{4-[2-(5-fluoro-2-{3-[(methylamino)methyl][1,2,4]triazolo[4,3-a]pyridin-6-yl}phenoxy)ethyl]-1,5-dimethyl-1H-pyrazol-3-yl}(morpholin-4-yl)methanone 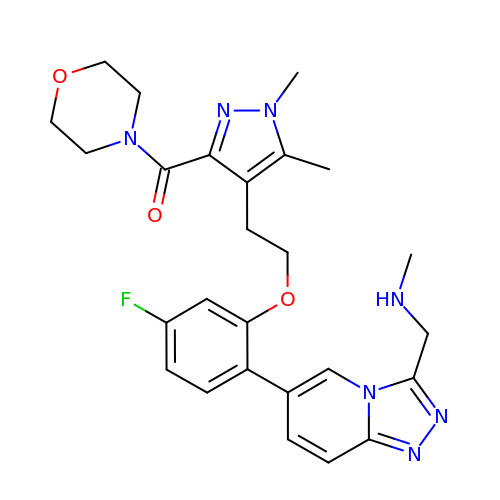| C26 H30 F N7 O3 | NIWAAHIPMDGEGU-UHFFFAOYSA-N>[2x]GSHMAIATINPTTGEICQRFKALTPAEIDAKLAKAQEAFQAYRRTSFSQRRQWLENAAAILERDTSKFAEIMTTEMGKTHQSAIAEAEKSALVCRYYAEHGEQFLANEYTETQATESYVCYQPLGILLAVMPWNFPFWQVFRFAAPALMAGNVAVLKHASNVPQCALAVEAILEAAGFPEGVFQTLLIGASQVEQVIKDPRVKAATLTGSEPAGASLASLAGQEIKPTL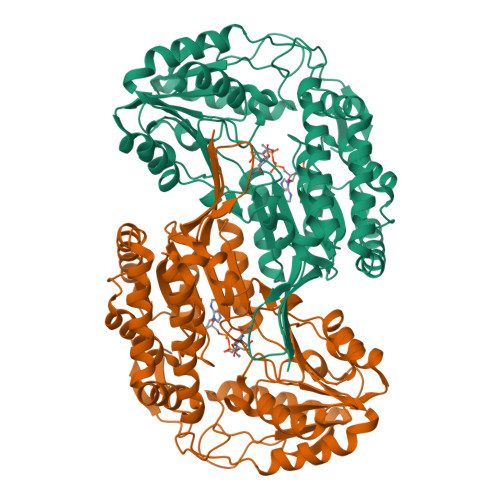LELGGSDPFVVFPSADLDEAVEVGTVARTMNNGQSAIAAKRFILHEAIAAEFLEKLHLKFASLKIGDPMAPETDIGPLATEGILQDISRQVDQAVAAGAKILLGGRPLDRAGYFYPPTILTEIPPGAKILQEELFAPVAMVFTVKDLDQAIALANDIPFGLGASAWTNDPAEQQRFIQELDAGAVFINGMVKSDPRLPFGGTKRSGYGRELGLAGIRTFVNAKTVWLK>QEVRRGDFVRNWQLVAAVPLFQKLGPAVLVEIVRALRARTVPAGAVICRIGEPGDRMFFVVEGSVSVATPNPVELGPGAFFGEMALISGEPWSAT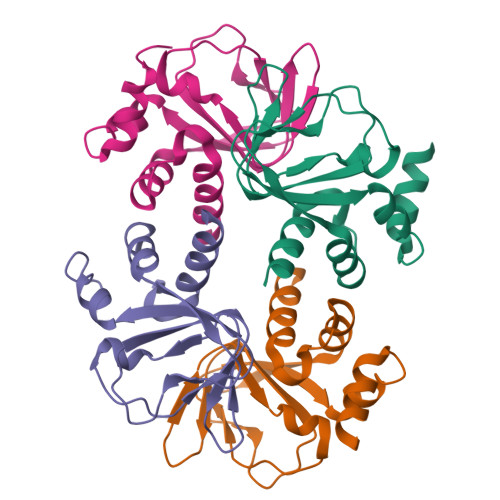VSAATTVSLLSLHSADFQMLCSSSPEIAEIFRKTALERRGAAASA[4x]N-(2-oxo-2,3-dihydro-1H-benzimidazol-5-yl)glycinamide | C9 H10 N4 O2 | 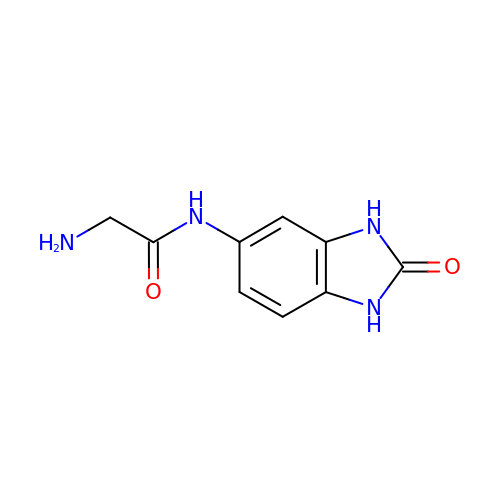VRPBYMLDIVHQOX-UHFFFAOYSA-N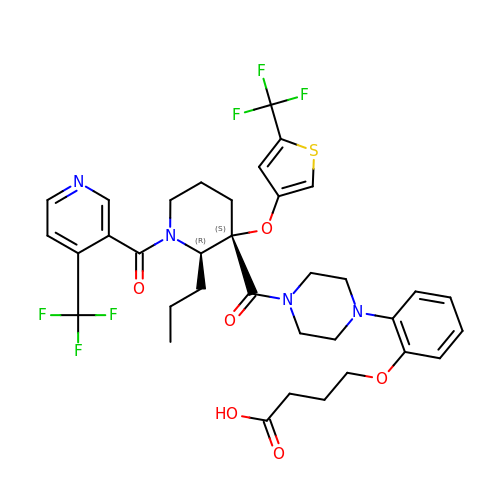4-[2-(4-{[(2R,3S)-2-propyl-1-{[4-(trifluoromethyl)pyridin-3-yl]carbonyl}-3-{[5-(trifluoromethyl)thiophen-3-yl]oxy}piperidin-3-yl]carbonyl}piperazin-1-yl)phenoxy]butanoic acid | C35 H38 F6 N4 O6 S | NWHQFQGJSWFQRZ-YDYNHKSESA-N> MAHHHHHHMVLNYFYPGTKTLKNKLGIMGYKQLEKRCKRNAKKVINSLRNEPLPETFDSSYLKYLHKRLFGSAFEWAGYTRDLSFAFDDGTIAQMSMMKIPGTDIYFAHGDKIQENLKEFDEILASKSNLQGLSREDFIEETVKLFSFLNYIHPFRAGNEAVQHIFFEKLAEAAGHKLDFSVVTEERIMRACNDAMALKGEEAHQAMKSLFEDISNPEEVIILRDFFKHIPRVERQRLNDE

Proteins containing a FIC domain catalyze AMPylation and other post-translational modifications (PTMs). Among these, Bartonella effector proteins (Beps) comprise a particularly diverse ensemble of FIC domains that subvert various host cellular functions. The FIC fold comprises eight conserved α-helices and encompasses a characteristic active site loop between helices α4 and α5 that forms most of the catalytic center and the substrate binding pocket. Additionally, FIC domains generally contain a β-hairpin between helix α2 and helix α3 that is referred to as the “flap” and mediates docking of a target segment in extended conformation via β-strand augmentation.

BepFIC domains with a glutamate (E159) in position G2 are represented by the B15_Bep8 and B11C_Bep8 structures, which are virtually identical. Although the motif is highly degenerated to PFxxGNE, the fold of the domain and, in particular, of the active loop are canonical. Nevertheless, the binding of a triphosphate-nucleotide appears to be impossible due to the presence of the side-chain in position G2 (compare Figure 9A and Figure 9B). However, simple outward rotation of the glutamate side-chain allows the accommodation of an AMPylated side-chain in a constellation very similar to that of the Tyr-AMP target side-chain in the IbpA/Cdc42 complex. Intriguingly, the model would allow binding of water molecule to the N-terminal end of α5 ready for a nucleophilic attack onto the phosphorous, which is in line with its phosphoester bond with the tyrosine, i.e., it is ready for deAMPylation of the modified side-chain. The strict conservation of a glutamate in G2 may then point to a role in water binding and proton abstraction, i.e., the glutamate would function as general base. About one quarter of BepFIC domains display a glutamate in the G2 position which would clearly interfere with the triphosphate-nucleotide binding mode observed in AMP transferases, i.e., with the γ-phosphate forming a salt-bridge with R2. However, binding of an AMPylated target to members of this group of BepFICs appears possible, which suggests that they might act as deAMPylases with the glutamate in G2 involved in binding and deprotonation of the hydrolytic water. B15_Bep8 Fic crystals were grown from a solution of 20% w/v PEG 8000, 0.1 M HEPES/NaOH, pH 7.5. Data for Bqu_BepC FIC, B15_Bep8 FIC, and Bcl_Bep5 FIC were collected at 100 K on a Rayonix MX-300 detector at a wavelength of 0.9786 Å on beamline 21-ID-G at the Advanced Photon Source (APS, Argonne, IL, USA).3-HYDROXYBENZOIC ACID | C7 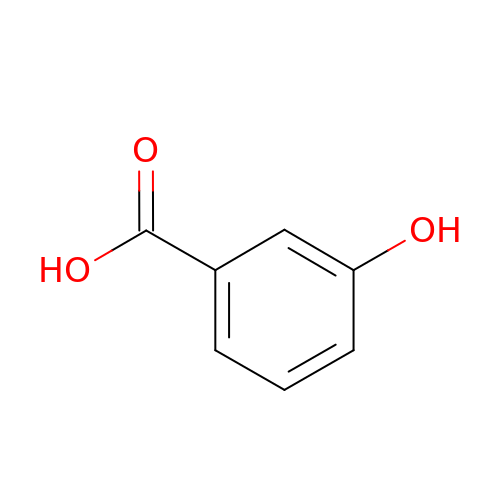H6 O3 | IJFXRHURBJZNAO-UHFFFAOYSA-N> GHMWSATNEEDDLSVEAEI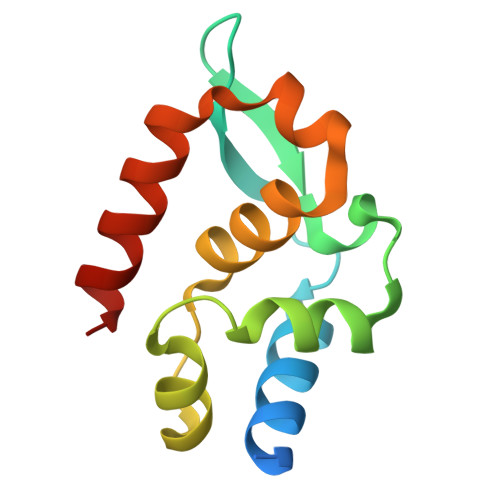AHQIAESFSKKYAFPSRSSGIFLYNFEQLKMNLDDIVKEAKNVPGVTRLAHDGSKLPLRCVLGWVALANSKKFQLLVEANKLNKIMQDDLNRYASC> Q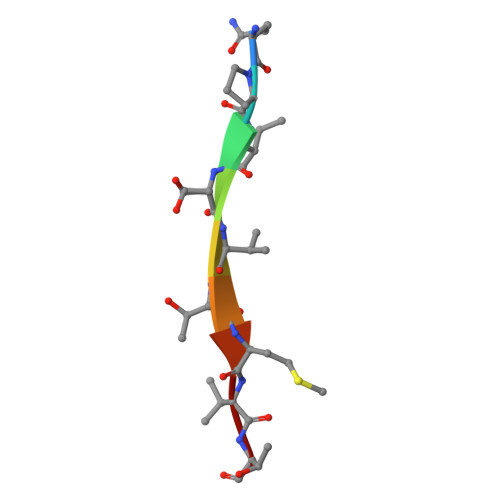PISVTMVT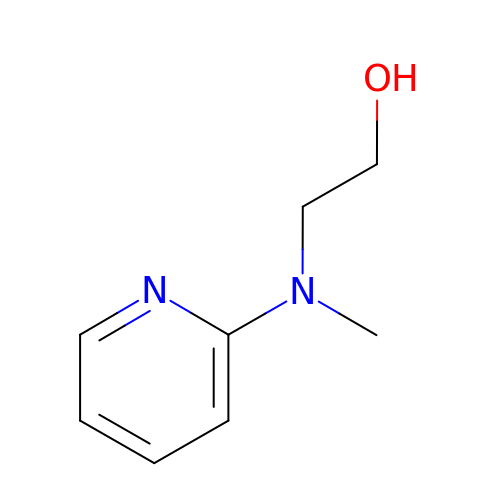2-[methyl(pyridin-2-yl)amino]ethan-1-ol | C8 H12 N2 O | MWGKOPUDDQZERY-UHFFFAOYSA-N> MSLEEFDEVKYDHSTKRLDTPSRYLLRKARRNPNGLQELRESMKSSTIYVGNLSFYTSEEQIYELFSKCGTIKRIIMGLDRFKFTPCGFCFIIYSCPDEALNALKYLSDTK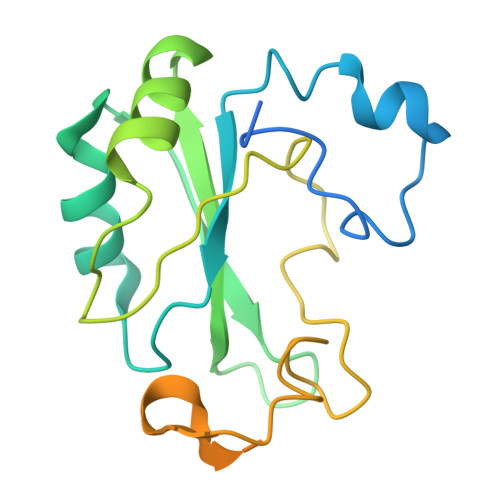LDEKTITIDLDPGFEDGRQFGRGKSGGQVSDELRFDFDASRGGFAIPFAERVGVPHSRFDNSSSQSNTNNYIPPPDAMGTFRPGFDEEREDDNYVPQ> QPDSVSIPITCCFNVINRKIPIQ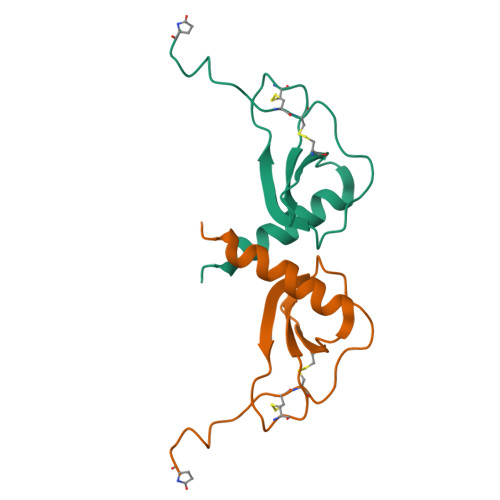RLESYTRITNIQCPKEAVIFKTQRGKEVCADPKERWVRDSMKHLDQIFQNLKP>[2x]MGSSHHHHHHSSGENLYFQGHMEAIQTHPANAAQAKAFTAPGSLSFPGGASEIANSTAPTNGASNGGQQQGVQATSGAGVTPATPAATPGAGPAGPSGITPTLQNIVATVNLDCRLDLKTIALHARNAEYNPKRFAAVIMRIREPKTTALIFASGKMVVTGAKSEDDSKLASRKYA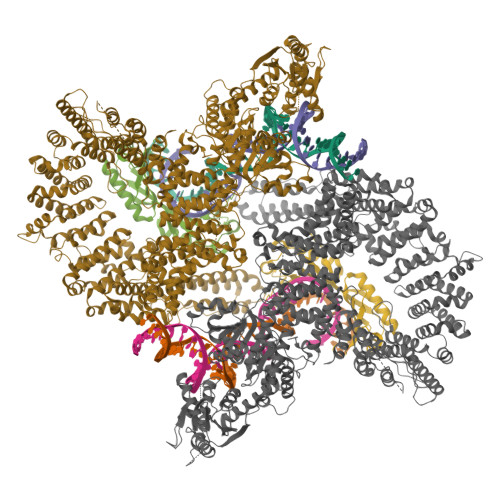RIIQKLGFNAKFTDFKIQNIVGSCDIKFPIRLEGLASKHHNFSSYEPELFPGLIYRMIKPKIVLLIFVSGKIVLTGAKVREEIYQAFEMIYPVLQDFRKV;>MATRLDRLVTILETGSTRLIRDTAVNQLADWQKQHPEELFNLLSRVVPYLRHKDWETRTTAAKAIGKIIENAPLYDPNAGQDEAAPEPTNGSFEVKKEEEKDVLEQDNFFRLESLDVATIVKYGRPLLRGGPVDYNLAALDPQKRLAHLKKTLNGRLGLLGRVFEDEEMPVEQIASPITPNDAAGANGVGRQDGASNDNQSQAIDESKMSARQLNVLKRKRKREAQKAAQGKSGFGDLSLRRSTTAGSDAFGEDTPMPDADSKKNKLAEYFSLDRPENTEEDTKIVSEFKGPVLPIKSEIEADDSLEGAEWPFERLCEFLKVDLFDPQWETRHGAAMGLREVIRVHGAGAGRRRGKTRKENNDLNRQWLDDLAYRLLCVLMLDKFTDYSSDTSVAPIRETVGQTLGAVLRHISVESVHAIYRLLYCMVTQEDLPSEQNMWAVCHGGMVGLRYVVAVRKDLLLQDGDMIDGVVRCVMQGLGDIDDDVRSVSAATLIPMAKEFVMMRRSALDSLINIVWESLSNLGDDLSASTGKIMDLLATLCSFPEVLEAMKVSASQDEERSFTLLVPRLYPFLRHTITSVRLAVLKALMTFANLGGETSQGWLNGRILRLIFQNIIVERDQDTLNMSLELWTTLVRRLAARDPAILADEFEAHAEPMMQLALHPIGVPRHPIPMNPALFQKPSGGTYSLPGASQTNSRRSSPPEGERATKRRRKSTKAEDVAPSTHTHDVDGHMIQGEVDLVGVDVLIRSRISAAKAMGLIMSFIPTPRLASYDTAVLQALSSPYASTQLAAAMVIDEYAKNCSTPEVASRFIEPLQKIIDLERPSHYRDLVTYVQRVRSASQQLINLFRDHGKVSQGKLPTLAVVVQGEPEAGPGAFSIANAEKVVNEDFERLKRLMAPGQRLIALPQLNEAREQTVEVIEEAKAAKEARDARIKAAAACALVAMKVLPKKPSPLIKAIMDSIKTEENQELQSRSAATIARLVQLFTESGRRGPAEKVVANLVKFSCVEVAETPEFPIHAHKTNVILSMQKEEDRVDHPDAVKYAREAKAARITRRGAKEALEILSKNFGAELLERVPTLRTFMEEPLVRAFSGDLPPEARDPENAFGQEIVDAMSVIRTMTPTLHPALHPFVMQQVPLVIKALRSDLSVFRYMAAKCMATICSVITVDGMTALVEKVLPSINNPLDLSFRQGAIEVIYHLIAVMGDAILPYVIFLIVPVLGRMSDSDNQIRLIATTSFATLVKLVPLEAGIPDPPGLSEELLKGRDRERTFIAQLLDPKKIEPFKIPVAIKAELRSYQQEGVNWLAFLNKYHLHGILCDDMGLGKTLQTICIVASDHHQRAEEFARTGAPEVRKLPSLIICPPTLSGHWQQEIKTYAPFLTVTAYVGSPAERRAMKDSLDKTDIVITSYDVCRNDIDVIEKYNWNYCVLDEGHLIKNPKAKITLAVKRLTSNHRLILTGTPIQNNVLELWSLFDFLMPGFLGAEKVFLDRFAKPIANSRYSKASSKEQEAGALAIEALHKQVLPFLLRRLKEEVLNDLPPKILQNYYCDLSDLQRKLFEDFTKREGKKITETAGRDDKEAKQHIFQALQYMRKLCNSPALVMKPGHKAYEDTQKYLAKHGTTLEDPIHAPKLGALRDLLVDCGIGVEGQESSDPLYTPIKPHRALIFCQMKEMLDMVQNTVLKQMLPSVSYLRLDGSVEANKRQDIVNKFNSDPSYDVLLLTTSVGGLGLNLTGADTVIFVEHDWNPQKDLQAMDRAHRIGQKKVVNVYRIITRGTLEEKILSLQRFKIDVASTVVNQQNAGLATMDTDQILDLFNLGESGPSLITDNKESIEAAAWSHPQFEK[2x]> MQLRKLLLPGLLSVTLLSGCAMDSVERVSLF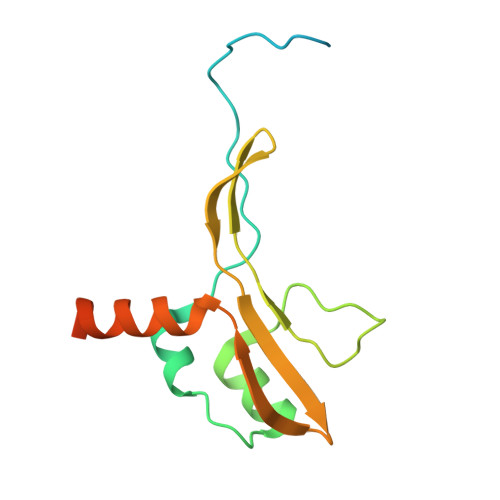PSYKLKIIQGNELEPRAVAALRPGMTKDQVLLLLGSPILRDAFHTDRWDYTFNTSRNGIIKERSNLTVYFENGVLVRTEGDALQNAAEALRAKQNADKQHHHHHHHHHH> MQYSIEKLKKEENSLAKDYYIYRLLEKNKISKKDAQDLNSHIFRYIGKIKSELEKIIPLKPYINPKYAKCYTYTANTILDANLTCQSVRLNSLVFIASLNSKDRTTLAQTFKNQRPDLTNLLLAFNTSDPMSYIVQKEDINGFFKLYNYSKKYDLDLNTSLVNKLPNHIGFKDFAQNIIIKKENPKFRHSMLEINPENVSEDSAFYLGVNALTYDKTELAYDFFKKAAQSFKSQSNKDNAIFWMWLIKNNEEDLKTLSQSSSLNIYSLYAKELTNTPFPKIESLNPSKKKNNFNMQDPFAWQKINKQIRDANASQLDVLAKEFDTQETLPIYAYILERKNNFKKHYFIMPYYDNIKDYNKTRQALILAIARQESRFIPTAISVSYALGMMQFMPFLANHIGEKELKIPNFDQDFMFKPEIAYYFGNYHLNYLESRLKSPLFVAYAYNGGIGFTNRMLARNDMFKTGKFEPFLSMELVPYQESRIYGKKVLANYIVYRHLLNDSI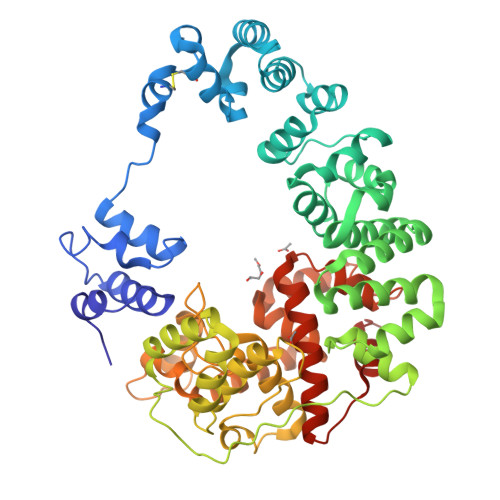KISDIFENLIQNKANDLNKS>MKKKDTCEIFGYDEEKVNRIQGDLQTVDISGVSQILKAIADENRAKITYALCQDEELCVCDIANILGVTIA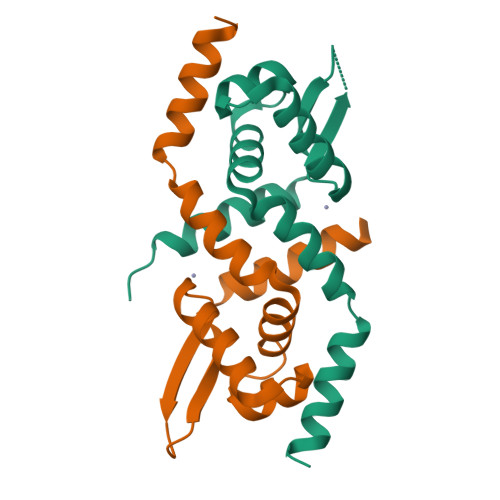NASHHLRTLYKQGVVNFRKEGKLALYSLGDEHIRQIMMIALAHKKEVKVNV[4x]>[2x]MNMTKYIPVLQSLLFVLLLSFSGHAQEHPSLILTKAGVEKIRAELGNIPIFDATLEKVKAEVDAEIALGIDTPLPKDYSGGYTHERHKRNFFILQKAGVLYQILNDEKYALYIKDMLFQYEGMYKDLPVHPQTRSYARGKLFWQCLNDSNWLVYVSQAYDCVYDYLSKKERKQLEKNLFRPFADYISIENPQFYNRVHNHSTWGNAAVGMIGLVMGDEELIQRALYGIEDDGLPIGAKDNDGGFIKVEGQKAGFLANIDEPFSPDGYYTEGPYAQRYAMYPFLIFAEALHNVRPQQKIFEHKDGVLLKSVNTLLSLSDADGEFFPLNDAQKGMSYHSRELVTAVDIAYHYGNHNPQLLSIAEEQGQVLLDDSGLAVALGIREGKSEDFQKKSIKLSDGA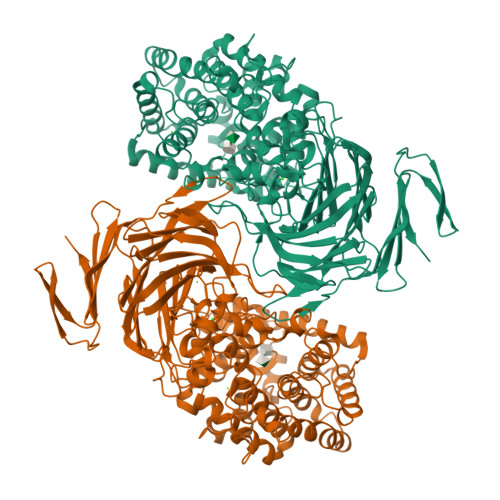NGDQGGVAILRYGNEAMTLVYKYAAQGLSHGHYDKLSFSLYEKGTEILQDYGLARFVNIEQKGGGNYLKENTTWAKQTIAHNTLVQNETSHFEGKYEVGSQHHSELYFFDASNPEVQVVSAKEQNAYPGTEMHRTMALIKTDGFEKPFVLDILRVGSNAANQYDLPFYFKGQVMQTNFDFTTPKSLEPLGSDNGYQHLWSEGLGQPKGDNSQLSWLENGRFYTLTTATNNDDELHFVRIGANDPEFNLRRDAGLIIRRKNTKNTTFVSILESHGHYSPVSEFSVNANSSISKIELMLDTKEYTAVLIDAKSNTEQTLLILANENKNVNKEHIIEIKGKEYRWTGPYQFIKIN>[4x]ATKKAVAVLKGTSNVEGVVTLTQEDDGPTTVNV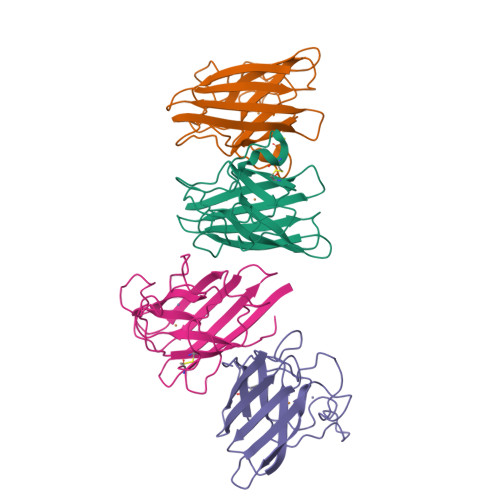RISGLAPGKHGFHLHEFGDTTNGCMSTGPHFNPDKKTHGAPEDEVRHAGDLGNIVANTDGVAEATIVDNQIPLTGPNSVVGRALVVHELEDDLGKGGHELSPTTGNAGGRLACGVVGLTPV> GPLGSSRLYLQNTAVMEELYRRNLSEDLVRDNGLSCGGREYWREPASTVGAASDGLSEEERRTAADAAERMTAVIAGTPGIAVERNVRDFRRGGWDVTPDNVESEFREVERRTFSDGVHWGRVIAFLAFSMSFAA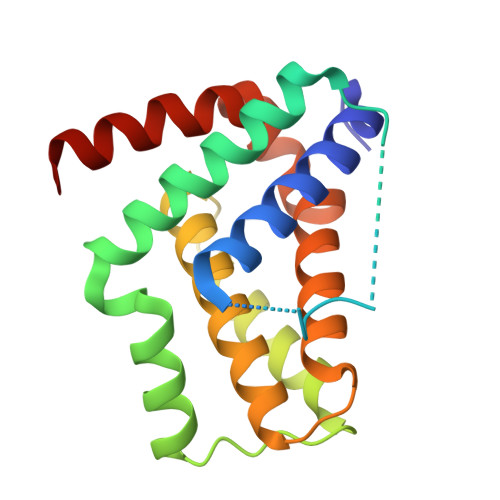YVNSRGIDGGAYSVFNWTLRVLNDSLADFIQRENGWRGFIVYADTLLRAQGS> ADVAGTSNRDFRGREQRLFNSEQYNYNNSLNGEVSVWVYAYYSDGSVLVINKNSQYKVGISETFKALKEYREGQHNDSYDEYEVNQSIYYPNGGDARKFHSNAKPRAIQIIFSPSVNVRTIKMAKGNAVSVPDEYLQRSHPWEATGIKYRKIKRDGEIVGYSHYFELPHEYNSISLAVSGVHKNPSSYNVGSAHNVMDVFQSCDLALRFCNRYWAELELVNHYISPNAYPYLDINN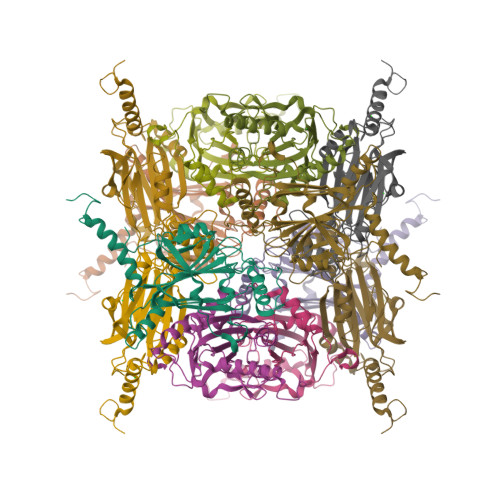HSYGVALSNRQ>[4x]MKTSIQQLVAV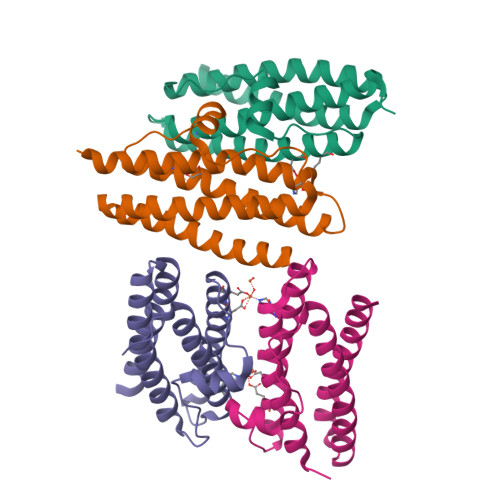LLNRQVANWVVLYVKLHNFHWNVNGPNFFTLHEKFEELYTEASGHIDTLAERVLSIGGSPIATLAASLEEASIKEATGGESAAEMVSSVVNDFVDLVGELKVARDVADEADDEATADMLDAIEAGLEKHVWMLEAFLE N~4~-methyl-N~4~-(3-methyl-1H-indazol-6-yl)-N~2~-(3,4,5-trimethoxyphenyl)pyrimidine-2,4-diamine | C22 H24 N6 O3 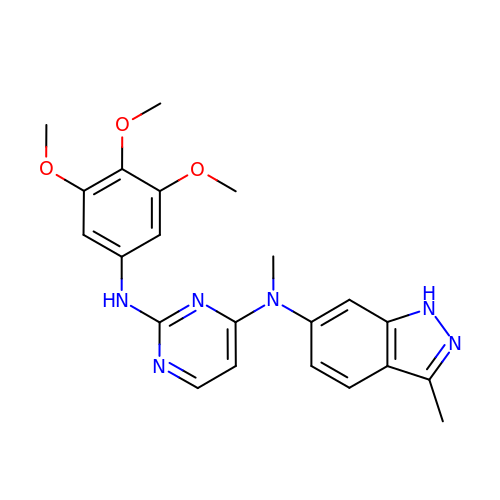| FLXGQDHYCWXTAI-UHFFFAOYSA-N>TEGSSPAYLKEILEQLLEAIVVATNPSGRLISELFQKLPSKVQYPDYYAIIKEPIDLKTIAQRIQNGSYKSIHAMAKDIDLLAKNAKTYNEPGSQVFKDANSIKKIFYMKKAEIEHHEMA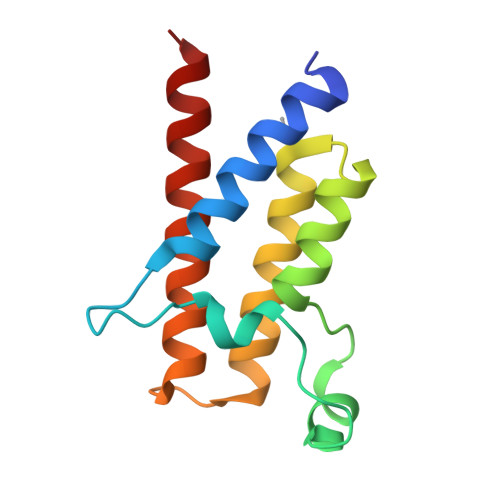[2x]In this route, ornithine is obtained from arginine by the action of arginase (arginine amidinohydrolase, ARGAH). Similarly to other eukaryotic (Di Costanzo et al., 2010) and prokaryotic (Bewley et al., 1999) orthologues, plant ARGAHs, are binuclear manganese metalloenzymes. Together with agmatinase, formiminoglutamase, and proclavaminate aminohydrolase, ARGAHs are grouped with the Ureohydrolase Superfamily.

In this work, ARGAHs from two model plant species, A. thaliana (AtARGAH1) and Medicago truncatula (MtARGAH), are structurally characterized by X-ray crystallography and small-angle X-ray scattering (SAXS). Based on the crystal structures of AtARGAH1 and MtARGAH complexes with ornithine combined with the analysis of sequence conservation of the key residues of plant ARGAHs their dual arginase/agmatinase function in plants is discussed.

>SNAMSTIARRGFHYMQRLNSANVSPALLEKAQNRVIDAALTFIRERAKFKGELMRSLGGVAATSSLLGVPLGHHSSFHEGSAFAPPRIREAIWCDSTNSTTEEGKNLRDPRVITNVGDVPIEEIRDCGVDDKRLANVISESVKLVMDEDPLRPLVLGGDHSISFPVVRAVSEKLGGAVDILHFDAHPDLYHDFEGNYYSHASPFARIMEGGYARRLVQVGIRSITNDVREQVKKYGVETHEMRTLSRDRPILENLKLGEGVKGVYVSIDVDSLDPSIAPGVSHHEPGGLLFRDILNILQNLQGDIVGGDVVEYNPQRDTYDGITALVAAKLVRELAAKMSK[12x]Human manganese superoxide dismutase (MnSOD) is a mitochondrial matrix metalloenzyme that catalyzes the dismutation of reactive superoxide radicals, generated as byproducts of mitochondrial respiration, into molecular oxygen (O2) and hydrogen peroxide (H2O2). As the only known mitochondrial enzyme capable of converting reactive radicals into diffusible products that can be further metabolized or exported, MnSOD serves as the critical first line of defence against oxidative stress. In the wild-type enzyme, Gln143 mediates proton transfers with the manganese-bound solvent (WAT1) to drive redox cycling of the metal, which is necessary for effective superoxide dismutation. Substitution with Asn stalls catalysis because the increased distance from WAT1 disrupts critical proton-coupled electron-transfer (PCET) events, and the redox cycling of the active-site metal is impaired.

In addition to H2O2 binding at the canonical LIG and PEO sites in the treated Gln143Asn enzyme, our results reveal a striking accumulation of five distinct cryo-trapped H2O2 molecules, either fully or partially occupying the space between the solvent-exposed enzyme surface and the Tyr34–His30 solvent gate. These new bulk-exposed peroxides, named Lb for Ligbulk binding sites, identified in this study have never been observed in any other peroxide-soaked MnSOD. To validate that the observed Lb densities truly correspond to H2O2 molecules, rather than misassigned or mobile waters, we performed a trial refinement in which we replaced each Lb peroxide in the treated structure with a fully occupied water molecule, as in the resting state. However, this does not satisfy the electron density, as shown by the appearance of positive Fo − Fc difference density around one of the missing O atoms in the trial structure. In addition to the Lb H2O2 molecules on the solvent-exposed surface, we observe H2O2 binding at the metal-ligated LIG position and at the PEO position at the mouth of the active-site solvent-funnel gateway between second-shell residues Tyr34 and His30. Overall, H2O2 treatment does not appear to significantly alter the active-site architecture of Gln143Asn MnSOD, except for the partial displacement of the manganese-bound solvent (WAT1) by a partially occupied (∼35%) H2O2 molecule bound at the LIG position, opposite His26.

>[2x]MKHSLPDLPYDYGALEPHINAQIMQLHHSKHHAAYVNNLNVTEEKYQEALAKGDVTAQIALQPALKFNGGGHINHSIFWTNLSPNGGGEPKGELLEAIKRDFGSFDKFKEKLTAASVGVQGSGWGWLGFNKERGHLQIAACPNNDPLQGTTGLIPLLGIDVWEHAYYLQYKNVRPDYLKAIWNVINWENVTERYMACKK> MSGKASTEGSVTTEFLSDIIGKTVNVKLASGLLYSGRLESIDGFMNVALSSATEHYESNN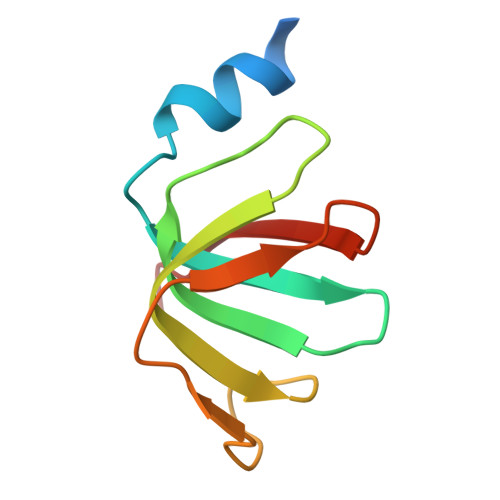NKLLNKFNSDVFLRGTQVMYISEQKI> MLPKRRRARVGSPSGDAASSTPPSTRFPGVAIYLVEPRMGRSRRAFLTGLARSKGFRVLDACSSEATHVVMEETSAEEAVSWQERRMAAAPPGCTPPALLDISWLTESLGAGQPVPVECRHRLEVAGPRKGPLSPAWMPAYACQRPTPLTHHNTGLSEALEILAEAAGFEGSEGRLLTFCRAASVLKALPSPVTTLSQLQGLPHFGEHSSRVVQELLEHGVCEEVERVRRSERYQTMKLFTQIFGVGVKTADRWYREGLRTLDDLREQPQKLTQQQKAGLQHHQDLSTPVLRSDVDALQQVVEEAVGQALPGATVTLTGGFRRGKLQGHDVDFLITHPKEGQEAGLLPRVMCRLQDQGLILYHQHQHSCCESPTRLAQQSHMDAFERSFCIFRLPQPGSWKAVRVDLVVAPVSQFPFALLGWTGSALFARELRRFSRKEKGLWLNSHGLFDPEQKTFFQAASEEDIFRHLGLEYLPPEQRNA

Pol μ is capable of performing gap-filling repair synthesis in the nonhomologous end joining (NHEJ) pathway. Compared with replicative DNA polymerase, Pol μ lacks proofreading activity, with an intrinsically high error rate of 10−3–10−5 for dNTP incorporation. Here, crystal structures and kinetics of Pol μ substituting dGTP for dATP on gapped DNA substrates containing templating T were determined and compared.

To further investigate the possible roles of these two residues in dGTP misincorporation, crystal structures of Q441A single-mutant and Q441A/K438A double-mutant proteins complexed with 1-nt gapped DNA and dGMPNPP were determined (Complexes 4 and 5, respectively). Although no crystal was obtained for the Pol μ single-mutant K438A, the structure of Q441A/K438A:DNA (Complex 5) revealed shared and distinctive features of dGMPNPP binding compared with the Q441A:DNA structure (Complex 4). While the templating T exhibited a further shift to an alternative conformation, dGMPNPP and the flipped 3ʹ-end dA of the primer strand in Complex 5 adopt a single conformation, similar to that observed in Complex 4. Compared with WT:DNA structures (Complexes 2 and 3), structures in which alanine was substituted for Gln441 (Complexes 4 and 5) exhibit a much more stable dGMPNPP, indicating that Gln441 may play a role in discrimination against dGTP misincorporation over the templating T on a 1-nt gapped DNA substrate. Notably, the Q441A/K438A double mutant displays a remarkably high misincorporation rate of dGTP vs. dATP (80.4 × 10−2). Steady-state kinetic measurements indicate that the K438A/Q441A double mutant has an overall misincorporation efficiency similar to that of the WT protein. Given that wobble T:dGMPNPP was observed in the structure of the double mutant (Complex 5), these two residues in the major and minor grooves appear to interact with the templating base and fine-tune the active site microenvironments of the incoming nucleotide binding.> MALRDFCSVDGSDLFWEWNVTWNTSNPDFTKCFQNTVLVWVPCSYLWVCFPFYFLYLSHHDRGYIQMTHLNKAKTALGFLLWIVCWADLFYSFWERSMGKLLAPVFLVSPTLLGITMLLATFLIQIERRRGVQSSGIMLTFWLIALLCALAILRSKIMTALKEDARVDVFRDVTFYIYFSLVLIQLVLSCFSDRSPLFSETINDPNPCPESSASFLSRITFWWITGMMVQGYRQPLESTDLWSLNKEDTSEQVVPVLVKNWKKECAKSRKQPVKIVYSSKDPAKPKGSSKVDVNEEAEALIVKCPQKERDPSLFKVLYKTFGPYFLMSFLFKAVHDLMMFAGPEILKLLINFVNDKKAPEWQGYFYTALLFISACLQTLVLHQYFHICFVSGMRIKTAVIGAVYRKALVITNAARKSSTVGEIVNLMSVDAQRFMDLATYINMIWSAPLQVILALYLLWLNLGPSVLAGVAVMVLMVPLNAVMAMKTKTYQVAHMKSKDNRIKLMNEILNGIKVLKLYAWELAFKDKVLAIRQEELKVLKKSAYLAAVGTFTWVCTPFLVALSTFAVYVTVDENNILDAQKAFVSLALFNILRFPLNI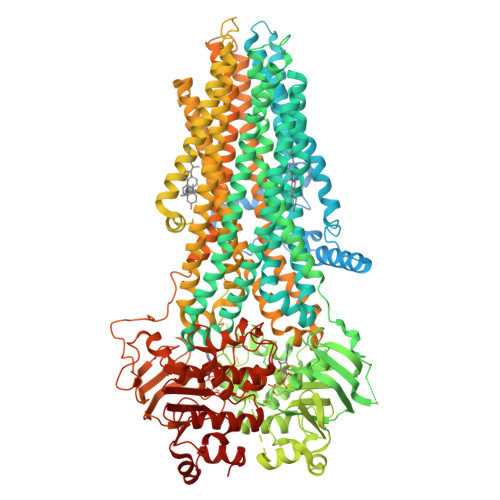LPMVISSIVQASVSLKRLRVFLSHEDLDPDSIQRRPIKDAGATNSITVKNATFTWARNDPPTLHGITFSVPEGSLVAVVGQVGCGKSSLLSALLAEMDKVEGHVTVKGSVAYVPQQAWIQNISLRENILFGRQLQERYYKAVVEACALLPDLEILPSGDRTEIGEKGVNLSGGQKQRVSLARAVYCDSDVYLLDDPLSAVDAHVGKHIFENVIGPKGLLKNKTRLLVTHAISYLPQMDVIIVMSGGKISEMGSYQELLARDGAFAEFLRTYASAEQEQGQPEDGLAGVGGPGKEVKQMENGMLVTDTAGKQMQRQLSSSSSYSRDVSQHHTSTAELRKPGPTEETWKLVEADKAQTGQVKLSVYWDYMKAIGLFISFLSIFLFLCNHVASLVSNYWLSLWTDDPIVNGTQEHTQVRLSVYGALGISQGITVFGYSMAVSIGGIFASRRLHLDLLHNVLRSPISFFERTPSGNLVNRFSKELDTVDSMIPQVIKMFMGSLFNVIGACIIILLATPMAAVIIPPLGLIYFFVQRFYVASSRQLKRLESVSRSPVYSHFNETLLGVSVIRAFEEQERFIRQSDLKVDENQKAYYPSIVANRWLAVRLECVGNCIVLFASLFAVISRHSLSAGLVGLSVSYSLQVTTYLNWLVRMSSEMETNIVAVERLKEYSETEKEAPWQIQDMAPPKDWPQVGRVEFRDYGLRYREDLDLVLKHINVTIDGGEKVGIVGRTGAGKSSLTLGLFRIKESAEGEIIIDDINIAKIGLHDLRFKITIIPQDPVLFSGSLRMNLDPFSQYSDEEVWTSLELAHLKGFVSALPDKLNHECAEGGENLSVGQRQLVCLARALLRKTKILVLDEATAAVDLETDDLIQSTIRTQFDDCTVLTIAHRLNTIMDYTRVIVLDKGEIQEWGSPSDLLQQRGLFYSMAKDSGLVSNSLEVLFQ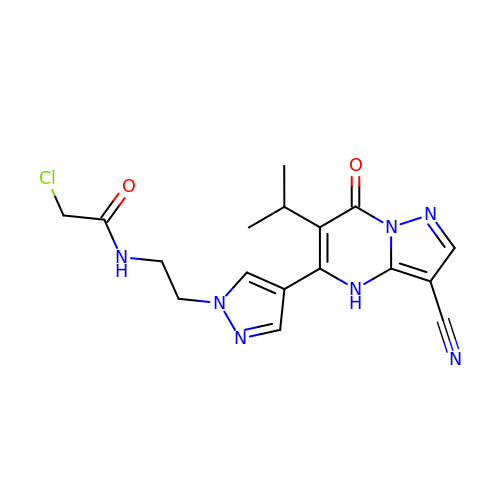2-chloranyl-~{N}-[2-[4-(3-cyano-7-oxidanylidene-6-propan-2-yl-4~{H}-pyrazolo[1,5-a]pyrimidin-5-yl)pyrazol-1-yl]ethyl]ethanamide | C17 H18 Cl N7 O2 | TUVMHEGGYLIJHD-UHFFFAOYSA-N> MDPPCTNTTAASTYLNNPYVRKALNIPEQLPQWDMCNFLVNLQYRRLYRSMNSQYLKLLSSQKYQILLYNGDVDMACNFMGDEWFVDSLNQKMEVQRRPWLVKYGDSGEQIAGFVKEFSHIAFLTIKGAGHMVPTDKPLAAFTMFSR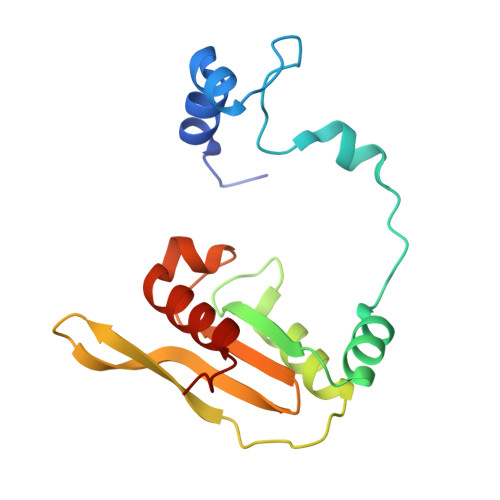FLNKQPYE>[4x]MDFSRNLYDIGEQLDSEDLASLKFLSLDYIPQRKQEPI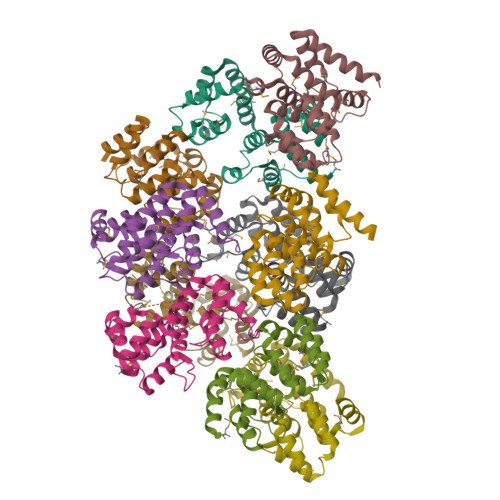KDALMLFQRLQEKRMLEESNLSFLKELLFRINRLDLLITYLNTRKEEMERELQTPGRAQISAYRVMLYQISEEVSRSELRSFKGGLQEEISKCKLDDDMNLLDIFIEMEKRVILGEGKLDILKRVCAQINKSLLKIINDYEEFSKER;>GSHMSAEVIGQVEEALDTDEKEMLLFLCRDVAIDVVPPNVRDLLDILRERGKLSVGDLAELLYRVRRFDLLKRILKMDRKAVETHLLRNPHLVSDYRVLMAEIGEDLDKSDVSSLIFLMKDYMGRGKISKEKSFLDLVVELEKLNLVAPDQLDLLEKCLKNIHRIDLKTKIQKYKQSVQGAGTS[6x]> GSPGIRLGSSEDNFARFVCKNNGVLFENQLLQIGLKSEFRQNLGRMFIFYGNKTSTQFLNFTPTLICADDLQTNLNLQTKPVDPTVDGGAQVQQVVNIECISDFTEAPVLNIQFRYGGTFQNVSVKLPITLNKFFQPTEMASQDFFQRWKQLSNPQQEVQNIFKAKHPMDTEITK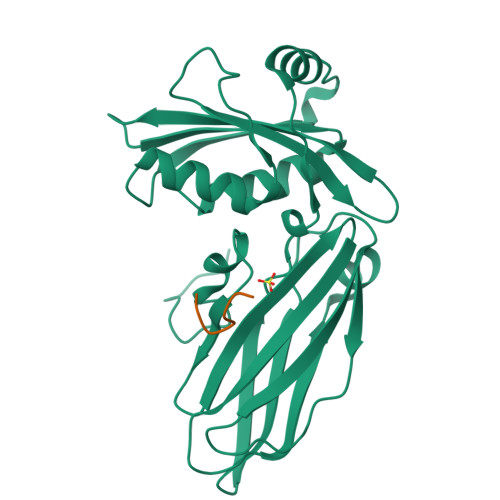AKIIGFGSALLEEVDPNPANFVGAGIIHTKTTQIGCLLRLEPNLQAQMYRLTLRTSKDTVSQRLCELLSEQF;> FSDPWGG> PIR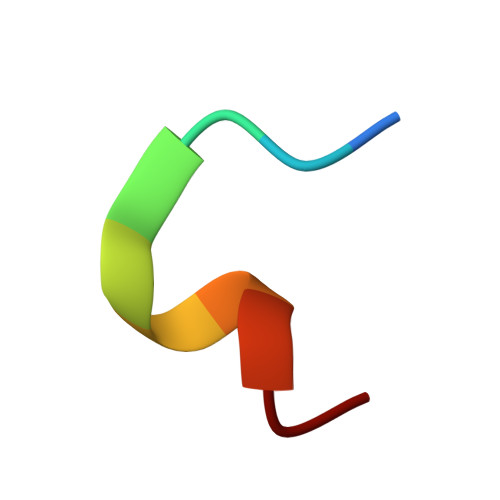YPWDVEC> GSMEIRVRVEKDPELGFSISG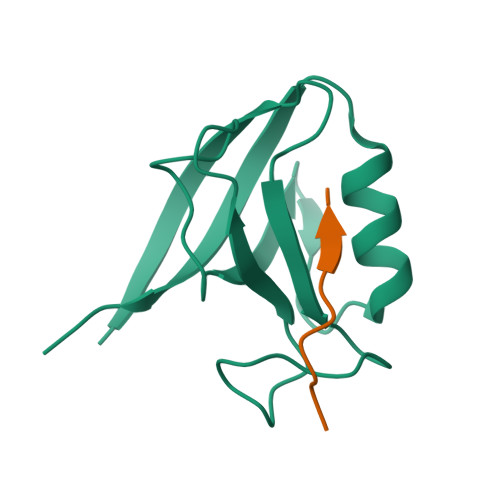GVGGRGNPFRPDDDGIFVTRVQPEGPASKLLQPGDKIIQANGYSFINIEHGQAVSLLKTFQNTVELIIVREVSS;> EYLGLDVPV> MLSSVVAP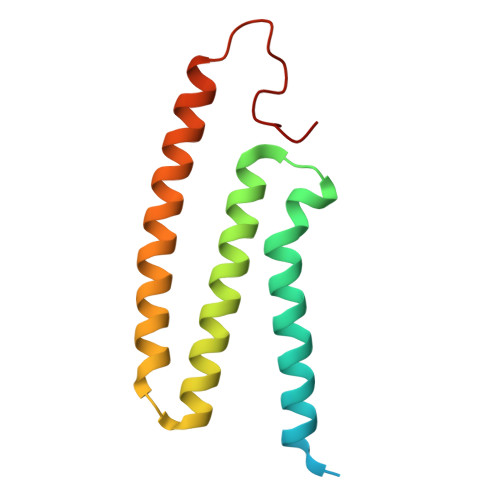QQPLSIAQPFAVRGYHNDAEFLGAVYNFSIRSVFITGILGAVYWRRNLITMLLCSEIAFIACSVNFLYASAYLNDMAGMLFSITITTISACETALGLALCVGYFQSRAANEVEALNLLK> MLRIKEVKKYNNRLGFPAGKEVRIRPLLEAGGFARGPIYVKYGRELSKHDPSSRSMAWNATVFDTALNHPTRPWTVTVVGGKKMVLGVRKEGLGFSEDDPPRSLNVKGGDDMADENYGGGNSTIVLVKSGGKDFAIGLDDLKELNSFGIGAGNGKLSLALGNPVNVLTGVVLPVEQRDGSVAYVAVNSDTKSVIYKVDAKGLQKNQKIDVNVRASAEKILLTKNNELLHISPQGLNVYSVQGSASTFKYFCPYFSSFGGWSRRFVDTVTLMDEGGNQEALIGTGPKGIEYMPVDEKCKNYVVEGVQDAKHAVVAPGATKEGNDIKVLGVYNGELCLLTLEVVDAVEPKLDQGSPAKPSAERVKATKSSKVTVRSGALSKPVSWLRDSLDEASFKNIVDKLSGKIRFSFPLVDLQGRMGLPIKLVVYYDESDGEDMSVLGRHWTLGRDCIVLDHGNTVFEDKQDYYLVKDQMKIRLERDWTKPSANGKVLFNMVGNKDATFEYTAREEKWEVSDGKIRYVYGMNNQGVVSVPGWADWYGPSANYDSKKIHSVQWNLVEISSVAHRDVKLKYTYTPLDPSTHTMHLLSITDDSNKTTIKFSYKTIEGLGKQVSSGLVKEHKFINNKLLEKVEIDSPSTAQVLKLTSTKIDSLYYLESIKQDDDPDPVLGFEYNKDDKLKPRVQQIRLPSKSVVDFKYTKQAIATQQFEQEIAKMADLYTGNEYSLEIEKTVGETDLYVRLKDSAGKNDFIKNQSIRIESYRGFKIKSYSPFMMHSYIAILVRYAEEKEKLHNKIYILNKGEDDSWKLDTTNNNSRVSEDKKFKYDFQEDSFVYYHSKKVHFEYKKSGTKVWSYTSKDIGDVDAFTLMNRGAVYCKNDLVLIRWDALGKLQQETLSDAKSKPSISDVDTFFEYIDVQGTFPEDEAEAKKEVDDYKRDLKESLSDYGLILYNNVVALRTIKLSFTGRITVKVLLYLLKHDYTVSSRSSIELQGGDLAKFNLTLDVFDEHKTKNTNDLDKYRFEFKKQGSKFKLTYIEATDKDNKPTKPSSQNEKLIGQYERRMKIPLDFEKYMMQVNQEGIIVNDHQIIHDNGNFIAKQLDRDTLKLTKFKIPLGAFSNFKKDSDGDEIKLCTKTEQERTESCVSLQTNSARNVSIKYPYYLVTQKKNDIKVLPLKINSRGWEDSVDYRGEILHGSSSHAAMVTTRMSDQKTIVRPLKALNKINKIYAQVISEEKLTTPYDSYVIKYEYEDPVVSMNQVAFKTTIVVPGGGKSATGYYRETNDLQDNQQIVQVMTADNQVFDPEYVKRMNEMQQEEDKQRDGAQLDAEQTITDKSGYHPILKTTPYSANQELVQFLGFEDYEDMTGWTVNKRPIQESNIRRNEFSATGRNFLLLKKGEELIAEFPNTAYYDNFIASTWIRTAQEATVGSTTDMLLLYVDNKPMKGTIKQSIDEWIYVEADSREIVVSESTTVKRVLFKIIVKSTGADDVHVDHVRLSPVNFNFEGSVYDARIGQRTATIQTNGFVSRRLYDAYNRRIAEVDETGNIKYLASYSKRVGNTKDEKKREGGYSSRIQMRAKHSWVESFSPYTMEKRWQIGGTATVEPNQAILQGQIISKEKFSSESICIRLVYSMSGSSQLSLTIGKTTVVVKPNAVQYKGHTATTPSNAELVIFATPKLTSIWVDGHLRIEAPETHAKFNNEAVSLQTSGPVGIKDVIVMEDAEIQVSYLNRDSKPLQEILLLDSSNVLIRQMMYDVIGRRVAETVWVQKSLIDGRSTAFKAFQYHDDFVSNDNPTDRNYFLNTGPMQGYVATATNTIYEGYPYSQTVYYNNPLEIRHKVGHPGVKNSIKGAFVHQYAIASDLAFIQRNYPKNEGYRQEEEKSPNGKKHVVVYNRRNKKVAEYTQVKDYNNILTTYIYDQHGNQIQMLPPSYYHEKSRSGDYQPEKQVVASPWAVTSKYDSTGEFITSKETPDGGRVEFIYNEYNQLRYQIHYKEDKQADKIVYFLYNIFGRMCEAGQVPANPTTLQQVRETTKSHQAIPNRDQAVYFDYGETESEPSLRGRIQRTVKKNKEVLFSEVMFFDEESNIIRKSYISPTTNETLSLVYLQENDKVSGIQYPFGVDGKQLILKYKHNLRGEIVEVARVEQKTSGQTEFIPIAGIDHDAEGKVTKISHNYGDSKFDQTYKYVAPGYLVEIANNFLTEKLYYTEKGYGCEPTGDGSILRTEFKASWHDKCDQNLIPLTARAFVSGGIDFTTAETCFDALLNLGYIDTTGRPVKTFYPDLETGLPMKCATPSNWRYISEKMLEQGYPEHYGHAYDYGSHGELIAAKSFVGKEKDSLTAPLSKASFANAGMKSHELDRFWDSLSRSINKVEGTKAIFEGTQQLTTGLVGSVIHKPKLESLLEGKGGDSSICTPWSSGDRTEEAKCKREYQQAFDKLKLKQVIQSLQEPVRKNVLRILKNTLASMLGNSPGDVESFSIDPNGNHGVFYTGFKRFELKYKHQKNQIATIKEGTKQQEKMIVHDDEGNVIKALHKKIDKIEYDPLTQRVSRIEMSDRSRTLEFGYDFRGERTFKRVRNKDNDIISVNYYVRDNKGNVLVEYKQEYPNPKDTNKPINTVTAYIHGPLGLLGFFRNNKYYNVLLDHEGSTRLVIHQGKVVAAYDYLPYGQMIRKYGSNPEAHIAFRYTGQEFDEETGLYNYHARLYDPDIGRFFQMDPMEQYASPYKYAGNSPVSQIDPDGQIAVTLVLMIIGAIVGAYLGAASANNSWNPAKWAWGDKKTWIGLFAGAIMGAFAVYGGAATFSYFTAMFGGSMIAGALATGVISVAGAFLGAAAASNQWNPAKWDWTSPAVWNGLLSGASIAVSFPSGFVGITRSFMSISSNLVKMIYASLMVGGFLLFVYLGGGMANNFNFQISQWDWKSPRTWFGMIEGASTIFMGTAGTAKHGAAKVYNVVKPNGLKMIWHKVNIPSKAFTMRRVKDTIILTWYKNGQSISKQILKTTVKADLAKIPKDFIMIHRGFFMPYQRIGYAAIAMPSMAGLMFKKNQYFFTNHPNGTLTKHVRKKRSAPMSSSAASPSVSNFLNDFFENMSELFDSFFSQTEHSHQDSQSSLSIGASYGRPSNESYHKSFQKLCYSPDSDGNQIICPQRESTVNIFSKGETFAPEAFGQDLFSRCLPLTWHDRPSIACDGEQTTFIYTPNQNIRVFDMVDGWLMLARIAPAALRNLKAGFSFLRDVVFSDEREQTVQVNDLSRCKQDLEVELLDLKRVMLKKQPNEVKWAQPILNDLEDDIGEFLSERKPSEKEFELLQERLSALREEIMENSSVATELNLSTLIGDMLKKMDGVNVGLNGDVRDMISTLSGMVPFSSSNLLA

One of the most abundant salivary proteins in Aedes aegypti mosquitoes is a high molecular weight (>300 kDa) protein called salivary gland surface protein 1 (SGS1); it is thought to have been acquired via horizontal transfer from bacterial endosymbionts. SGS1 is exclusively expressed in the salivary glands of adult female mosquitoes, which suggests that SGS1 is involved in blood-feeding and pathogen transmission. Here, we determine the native structure of SGS1 by the cryoID approach, showing that the 3364 amino-acid protein has a Tc toxin-like Rhs/YD shell, four receptor domains, and a set of C-terminal daisy-chained helices.

Cryo-EM images were obtained from salivary gland extracts without fractionation. The SGS1 structure is cocoon shaped, with dimensions of 210 Å × 115 Å × 86 Å. It is organized into 6 domains: two β-propeller domains, a rearrangement hotspot/tyrosine-aspartate (Rhs/YD)-repeats domain, a carbohydrate-binding module (CBM), a lectin carbohydrate-recognition domain (lectin-CRD), and a wedge domain. The C-terminal moiety, a ~230 aa-long sequence previously predicted to form a set of TM helices, is surprisingly almost fully buried within the chamber inside the cocoon shell and forms daisy-chained helices, which extend across the entire internal space to an opening at the middle of the Rhs/YD-repeats domain. DALI search of the Rhs/YD-repeats domain identified two top-ranking folds: Tc toxin and teneurin. Side-by-side comparison of these structures revealed that the SGS1 Rhs/YD-repeats domain is nearly identical to that in the BC components of bacterial Tc toxins and highly similar to that of eukaryotic teneurins, though the latter has a much shorter N-terminal β-sheet (cyan in Fig. 2b). Sequence alignment indicated that SGS proteins and Tc toxin contain all three residues required for catalysis (one Arg followed by two catalytic Asp), but teneurin lacks the last catalytic Asp, suggesting that SGS proteins are likely the AP with the corresponding auto-cleavage site located between residues 2733-2734 in SGS1. Nonetheless, the last catalytic residue of SGS1 (Asp2729) is pulled farther away from the catalytic center than that (Asp674) in Tc toxin. These observations suggest that a major conformational change must occur in SGS1 to activate its catalytic activity during its secretion from the gland to saliva. The exterior surface of the SGS1 Rhs/YD shell is decorated by five domains: β-propeller 1 (residues 1–344), β-propeller 2 (residues 705–1216), a carbohydrate-binding module (CBM: residues 1345–1494), a lectin carbohydrate-recognition domain (lectin-CRD: residues 1575-1715), and a wedge domain (residues 2225–2304, 2326–2465). Unlike the β-propeller 1 domain, the β-propeller 2 domain is located on the other end of the Rhs/YD shell and differs from the canonical β-propeller in three major aspects: distorted arrangement of its nine blades, insertion of a protruding lid atop the blades, and an occupied central tunnel.> ANPLYQKHIISINDLSRDDLNLVLATAAKLKANPQPELLKHKVIASAFFEASTRTRLSF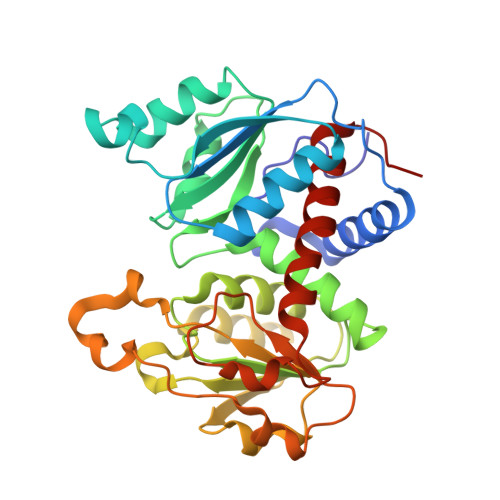ETSMHRLGASVVGFSDSANTSLGKKGETLADTISVISTYVDAIVMRHPQEGAARLATEFSGNVPVLNAGDGSNQHPTQTLLDLFTIQETQGRLDNLHVAMVGDLKYGRTVHSLTQALAKFDGNRFYFIAPDALAMPQYILDMLDEKGIAWSLHSSIEEVMAEVDILYMTRVQKERLDPSEYCNVKAQFVLRASDLHNAKANMKVLHPLPRVDEIATDVDKTPHAWYFQQAGNGIFARQALLALVLNRDLVL> MVYPQPKVLTPSRKDVLVVTPWLAPIVWEGTFNIDILNEQFRLQNTTIGLTVFAIKKYVAFLKLFLETAEKHFMVGHRVHYYVFTDQPAAVPRVTLGTGRQLSVLEVGAYKRWQDVSMRRMEMISDFSERRFLSEVDYLVSVDVDMEFRDHVGVEILTPLFGTLHPSFYGSSREAFTYERRPQSQAYIPKDEGDFYYMGAFFGGSVQEVQRLTRACHQAMMVDQANGIEAVWH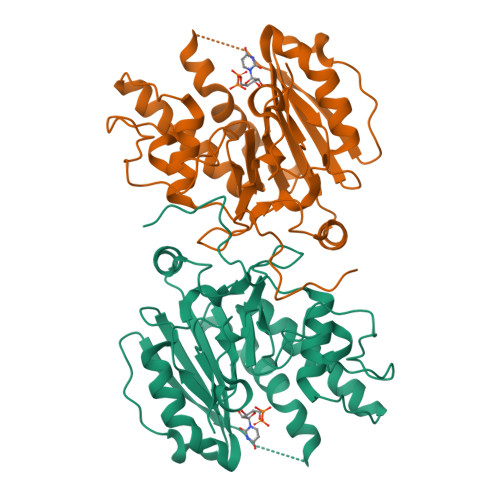DESHLNKYLLRHKPTKVLSPEYLWDQQLLGWPAVLRKLRFTAVPKNHQAVRNPE>MGSSHHHHHHSSGENLYFQGSHMVAVKGEGKKPAKKWATVEISKADEALRYYSAQGYTLLNNYLRDRPYKQREAIDTLLSRSYLNDEPTSAGEFDKAMKAYVADVEAGLAKLPASPELSFVYRGLALDKPELAALKEQFTGVGNIVVEPGFMSTSPDKAWVNDTLLKIRLPAGHGGRLLGDAAHFKGEAEMLFPTQTRLRVDRVVSSTSGD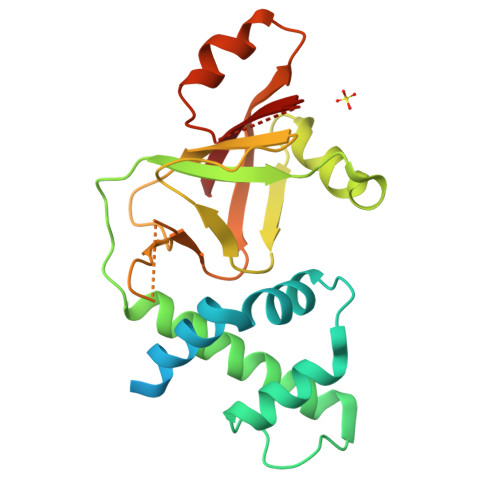FDTLLNTIPTSDNASDNRNRIKRLIEVSVL[2x]>[2x]ATETSFNFPNFHTDDKLILQGNATISSKGQLQLTGVGSNELPRVDSLGRAFYSDPIQIKDSNNVASFNTNFTFIIRA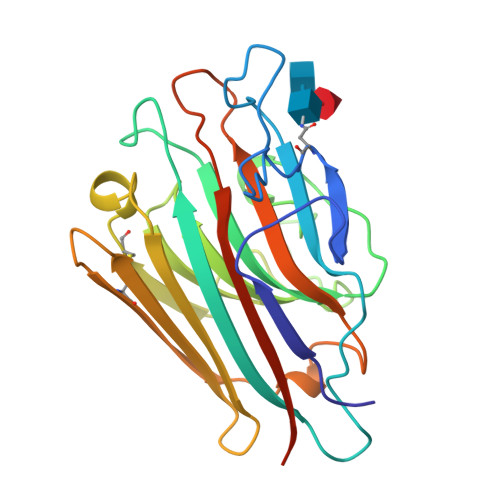KNQSISAYGLAFALVPVNSPPQKKQEFLGIFNTNNPEPNARTVAVVFNTFKNRIDFDKNFIKPYVNENCDFHKYNGEKTDVQITYDSSNNDLRVFLHFTVSQVKCSVSATVHLEKEVDEWVSVGFSPTSGLTEDTTETHDVLSWSFSSKFRNKLSNILLNNIL> SDLDRCTTFDDVQAPNYTQHTSSMRGVYYPDEIFRSDTLYLTQDLFLPFYSNVTGFHTINHTFDNPVIPFKDGIYFAATEKSNVVRGWVFGSTMNNKSQSVIIINNSTNVVIRACNFELCDNPFFAVSKPMGTQTHTMIFDNAFNCTFEYISDAFSLDVSEKSGNFKHLREFVFKNKDGFLYVYKGYQPIDVVRDLPSGFNTLKPIFKLPLGINITNFRAILTAFSPAQDTWGTSAAAYFVGYLKPTTFMLKYDENGTITDAVDC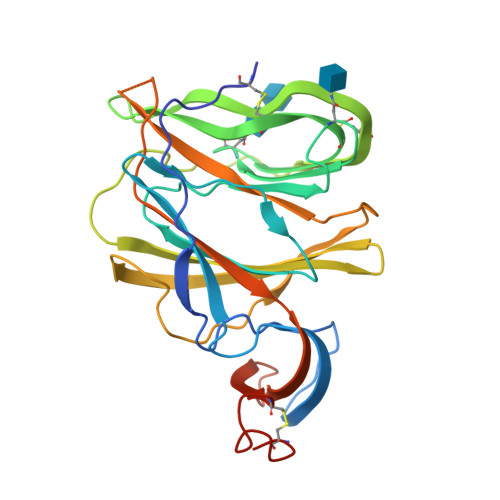SQNPLAELKCSVKSHHHHHH>[5x]TKKSREEIVKEILGRANPNNIPIVDEQPVKVSFKYSLQDIYTADVGTDQVELGLWLVISWKDRSLSWSNECTTFNELTLPSKYIWLPHIEVYNSIGKPGIHSDQLVRVYKDGTVTFVPQYTIRFSCALENVTTEQGAACTLKFGPWTYDVRDLVLDESQQVDLTTYAGGERFQLIEAKQKVNKKTYPCCPQSFEDIELRVTFKKI

Acetylcholine-binding proteins (AChBP) have been described in several gastropods and, more recently, also in an annelid. They are homo-pentamers and water soluble homologues of the extracellular, pentameric ligand-binding domain (LBD) of the membrane-bound nicotinic acetylcholine receptors (nAChR) that belong to the Cys-loop receptor superfamily. In AChBP, the pentameric quaternary structure and the overall subunit features of nAChR-LBD are fully conserved; this also includes the typical pocket-like active site at the five inter-subunit interfaces, with several strictly conserved aromatic residues for ligand binding, and a C-loop for controlled access to the active site. We retrieved full-length sequences of two distinct subunits (termed BgAChBP1 and BgAChBP2), encompassing 205 amino acids plus signal peptide and sharing 52% sequence identity. The resulting cryo-EM structure is a regular pentagonal dodecahedron ∼22 nm in diameter and assembled from twelve ring-like pentamers; each pentamer measures 7–8 nm in height and width and comprises a central channel that is ∼2 nm in diameter.

We docked twelve copies of the homology-modeled BgAChBP1 pentamer into the 6-Å cryo-EM structure. Comparable results were obtained with the BgAChBP2 pentamer (not shown). In BgAChBP2, the putative disulfide bridge C16↔C64 is lacking, but residues D25, R63 and E70 are conserved. R2, R3, D26 are substituted for K2, K3, E26, but these isofunctional exchanges suggest the same role in inter-pentamer binding. Instead of phenylalanine F71, the single cysteine C71 is present in BgAChBP2. The only possibility for this covalent dimerization exists via C71↔C71, since the other four cysteines in BgAChBP2 form the canonical disulfide bridges in loop L7 and loop L10. In silico, we assembled a BgAChBP2 homo-dodecahedron, with three C71 in the center of each vertex (not shown). However, such a particle might not exist in vivo, because we could not produce it from recombinant BgAChBP2. Recombinant BgAChBP2 formed many pentamers, indicating that the protein refolding was successful, while rosette-like particles were completely absent. Alternatively, BgAChBP2 might exclusively form di-pentamers, with C71↔C71 bridges as covalent linkers.> GAMGSGIQRPTSTSSLVAAAMAEEEEVEEGRSSSSAILDLPEPLLLHILSFLTDVRSRHRAALACGRMRAAERATRSELSLRGDPRSPGFLFLSHAFRFPALEHLDLSLVSPWGHPLLSSVPPCGGGGGGAPSASSSSGMNVYHPEAISEQNAFIAARLAGCFPAVTSLAVYCRDPTTLANLTPHWQASLRRVKLVRWHQRPPTLPDGADLEPLLETCAALRELDLSEFYCWTEDVVRALTTHPSATAALTHLDLGLAAATDGFKSSELGPIAASCPNLRKLVAPCLFNPRFSDCVGDDALLSLATSCPRLTVLRLSEPFEAAANIQREEAAITVAGLVAFFAALPALEDFTMDLQHNVLEAAPAMEALARRCPRIKFLTLGSFQGLCKASWLHLDGVAVCGGLESLYMKNCQDLTDASLAAIGRGCRRLAKFGIHGCDLVTSAGIRRLAFTLRPTLKEVTVLHCRLLHTAECLTALSPIRDRIESLEINCVWNTTEQPCSVANGTTTECDPEDDELGEVYESAAKKCRYMEFDDLGSWEMLRSLSLWFSAGQLLSPLISAGLDSCPVLEEISIKVEGDCRTCPRPAPRTIFG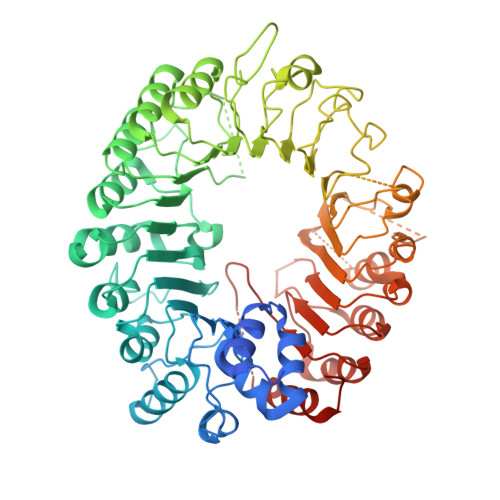LSDLAGFPVLAKMKLDLSEAVGYALTAPTGQMDLSLWERFYLHGIESLQTLYELDYWPPQDKDVHHRSLTLPAVGLIQRCVGLRKLFIHGTTHEHFMTFFLSIPNLRDMQLREDYYPAPENDLMFTEMRAESWLRFEVQLNSRQIDD>VCSCRLVFCRRTELRV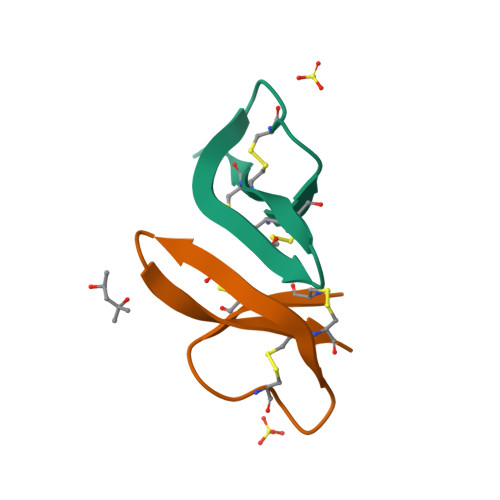GNCLIGAVSFTYCCTRV[12x]>HHHHHHMPRSVTADASGSFLTLTFEDGSESRFHAIWLRDNALDPETRSPGNGQRLITIGDIPADTRISTALVDDGALTVTFAPEGKTVTFPGKWLKSNAYDTDQSSEVGRTSPDVETWDSSQPAPAFDWNEVQSDPKAKRDWLDAIARLGFAKLVNGPVREGALIECASMFGFVRETNYGKYFEVRTEVNPTNLAYTGLGLQAHTDNPYRDPVPSLQILYCLENSAEGGDSIVVDGFRAAERLRDEDPEGFALLAGNPARFEYKGSDGVHLRARRPMIELSPDGEMIAIRFNNRSSAPFVDIPFEKMEAYYAAYRRLGEFIDDPEMGVSFKLEPGESFIVDNTRVLHARLGYSGSGSRWL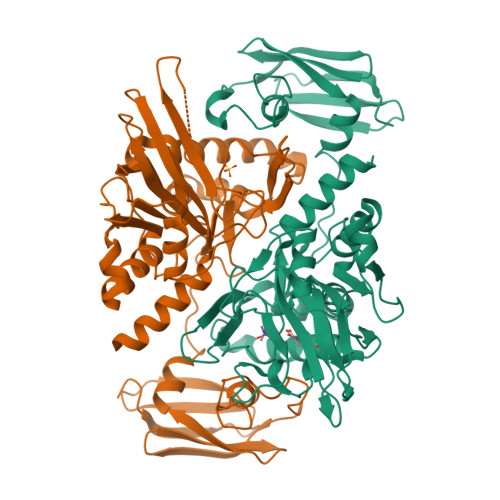QGCYADKDGLFSTLNVLNAQLGG[2x]9,9,9-tris(fluoranyl)-8,8-bis(oxidanyl)-~{N}-phenyl-nonanamide 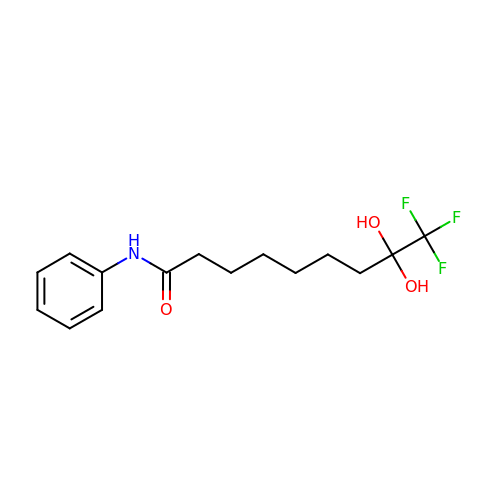| C15 H20 F3 N O3 | DOVGAPNVSPZBAT-UHFFFAOYSA-N>AHSPLQSSIQEKILTARPGDYAVLSRGSQKFFFLIRQSSSEATWVEMSEFASLTQQEKKLVEQSSWKNAFHQLQSSKKVYLLRISKNPLMIFVLKNAQWMPLSEKDPLPFFVKILRLPLSPAPSHLIKYKGKERTPWSPRTSLNGELITLPSSAWISVWPKDS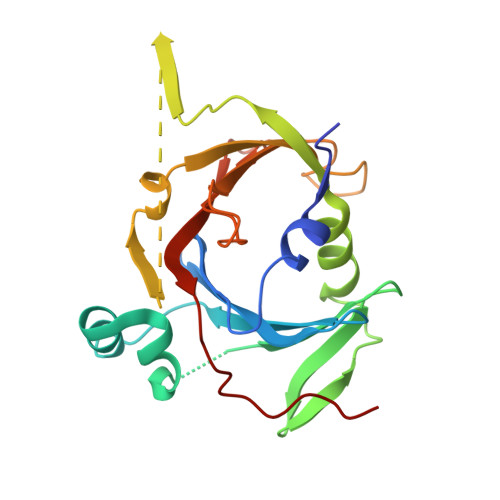SPLSEKNILIYFSNNERLAFPLWTSIDTPTGTVIIKTIEMGHQAASSYPALPNF[2x]> MSPVDFKDKVVIITGAGGGLGKYYSLEFAKLGAKVVVNDLGGALNGQGGNSKAADVVVDEIVKNGGVAVADYNNVLDGDKIVETAVKNFG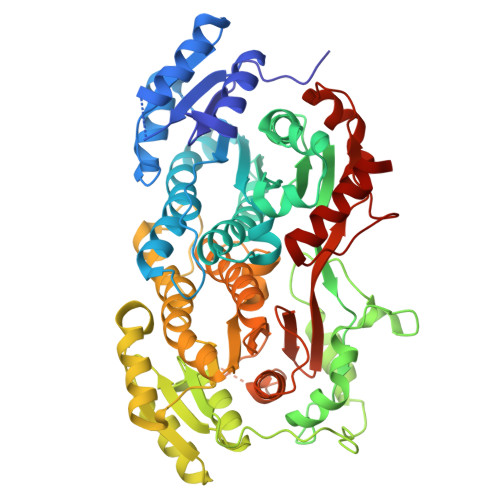TVHVIINNAGILRDASMKKMTEKDYKLVIDVHLNGAFAVTKAAWPYFQKQKYGRIVNTSSPAGLYGNFGQANYASAKSALLGFAETLAKEGAKYNIKANAIAPLARSRMTESIMPPPMLEKLGPEKVAPLVLYLSSAENELTGQFFEVAAGFYAQIRWERSGGVLFKPDQSFTAEVVAKRFSEILDYDDSRKPEYLKNQYPFMLNDYATLTNEARKLPANDASGAPTVSLKDKVVLITGAGAGLGKEYAKWFAKYGAKVVVNDFKDATKTVDEIKAAGGEAWPDQHDVAKDSEAIIKNVIDKYGTIDILVNNAGILRDRSFAKMSKQEWDSVQQVHLIGTFNLSRLAWPYFVEKQFGRIINITSTSGIYGNFGQANYSSSKAGILGLSKTMAIEGAKNNIKVNIVAPHAETAMTLSIMREQDKNLYHADQVAPLLVYLGTDDVPVTGETFEIGGGWIGNTRWQRAKGAVSHDEHTTVEFIKEHLNEITDFTTDTENPKSTTESSMAILSAVGGD>GPGSEFSLDHSDLVAELLKELSNHNERVEERKIALYELMKLTQEESFSVWDEHFK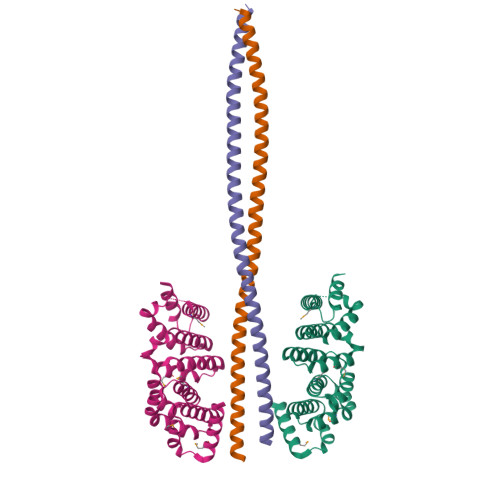TILLLLLETLGDKEPTIRALALKVLREILRHQPARFKNYAELTVMKTLEAHKDPHKEVVRSAEEAASVLATSISPEQCIKVLCPIIQTADYPINLAAIKMQTKVIERVSKETLNLLLPEIMPGLIQGYDNSESSVRKACVFCLVAVHAVIGDELKPHLSQLTGSKMKLLNLYIKRAQTGS[4x];>GPGSTTALQEALKEKQQHIEQLLAERDLERAEVAKATSHVGEIEQELALARDGHDQHVLELEAKMDQLRTMVEAADREKVELLNQLEEEKRKVEDLQFRVEEESITKGDLE[4x]> AVANATELVNKISENCFEKCLTSPYATRNDACIDQCLAKYMRSWNVIS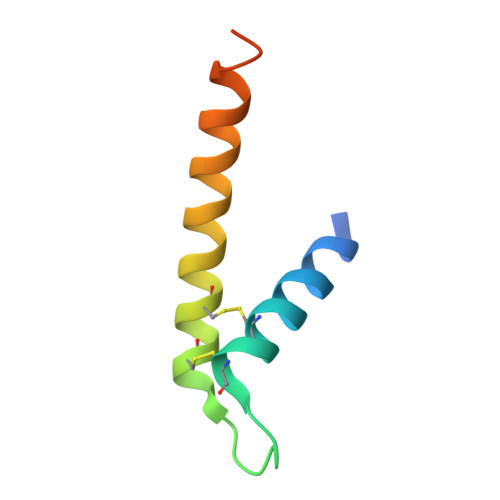KAYISRIQNASASGEI>[2x]MTARNPLEAQAWALLEAVYDPELGLDVV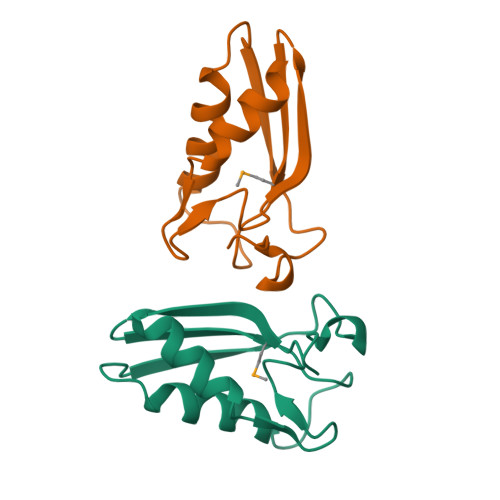NLGLIYDLVVEPPRAYVRMTLTTPGCPLHDSLGEAVRQALSRLPGVEEVEVEVTFEPPWTLARLSEKARRLLGWG> CGCGAA;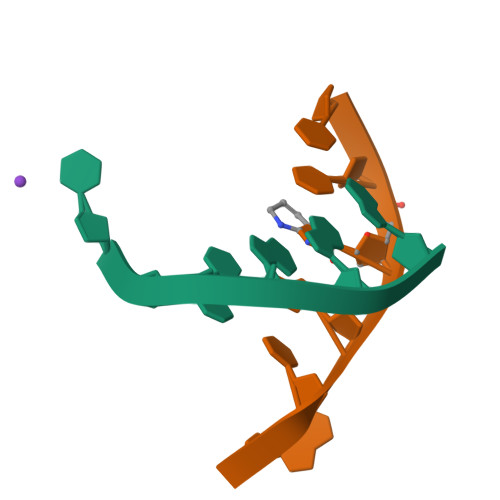> TTXGCG> SNAMKIIFSASPANRAAAYALRQAVFVEERGISADVEFDVKDTDQCEYAVLYLQPDLPITTLRLEPQADHVMRFGRVCTRKAYRGHGWGRQLLTAAEEWATQRGFTHGEIHGELTAQRFYELCGYRVTAGPYDE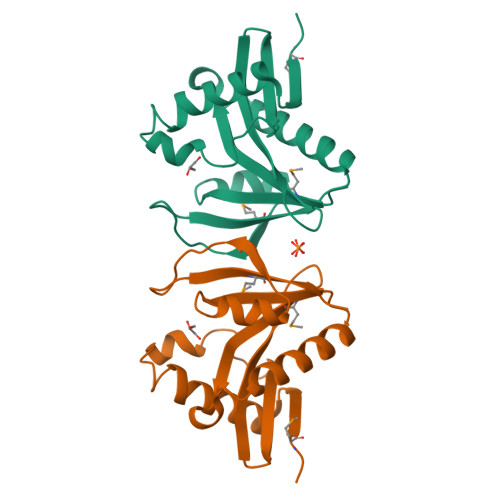DGAPVVIMHKQLL>HMPRVLVTGALGQIGTDLSLALRDKFGADSVLVSDVVEPGAKHPLAGLKGVEKLDCLDSNGFEKLVKEFKPTWMYHLPAIMSVRGEAEPDLAMDINVNTTRYALELARKYNIRIFIPSTIAAFGDKCGKTMTKDDTIMNPSTVYGVTKVYTELLGTWYRQKYGVDFRSVRLPGIISAATLPGGGATDYAIHMYHSALLQKKCVCPVLPYESLPMMYMPDTLNSLVKIMEAPLEKLTRTVYNITGFSFSPSELRFSIERCT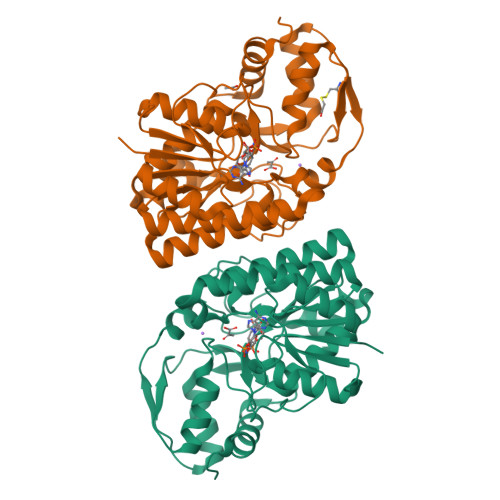DRTIEVEYVEGPAQKIANSWPDSLDDSNARNDWGHQVKYDIDMMSEDMLRQIPILHGLPSL[6x]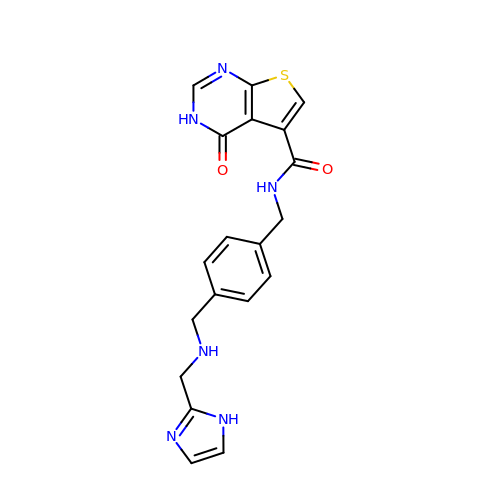N-(4-{[(1H-imidazol-2-ylmethyl)amino]methyl}benzyl)-4-oxo-3,4-dihydrothieno[2,3-d]pyrimidine-5-carboxamide | C19 H18 N6 O2 S | RLANZYKQCHLLJS-UHFFFAOYSA-N3-{[benzyl(ethyl)carbamoyl]amino}-5-(4-phenoxyphenyl)thiophene-2-carboxylic acid | C27 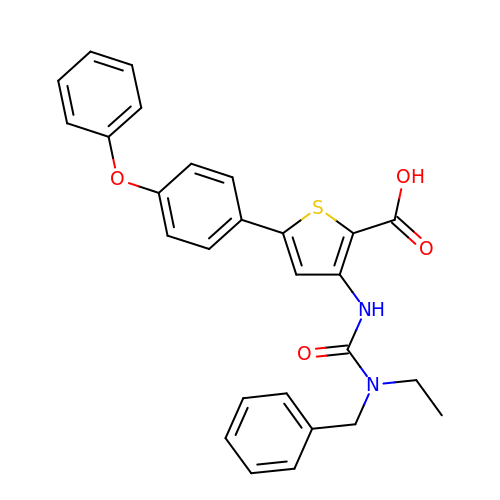H24 N2 O4 S | QMFIMKMXDIPTKO-UHFFFAOYSA-N> ATKDKK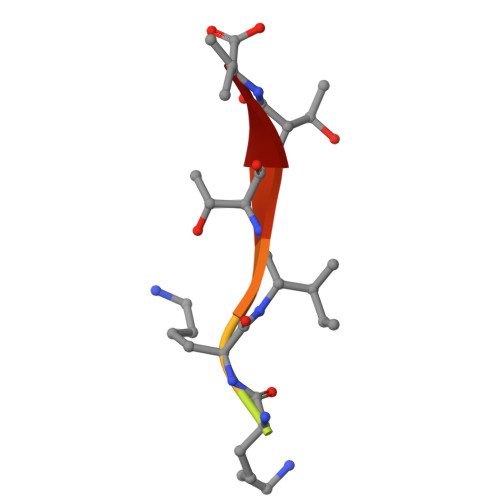ITTV> MGAKLAKTLQRFENKIKAGDYYEAHQTLRTIANRYVRSKSYEHAIELISQGALSFLKAKQGGSGTDLIFYLLEVYDLAEVKVDDISVARLVRLIAELDPSEPNLKDVITGMN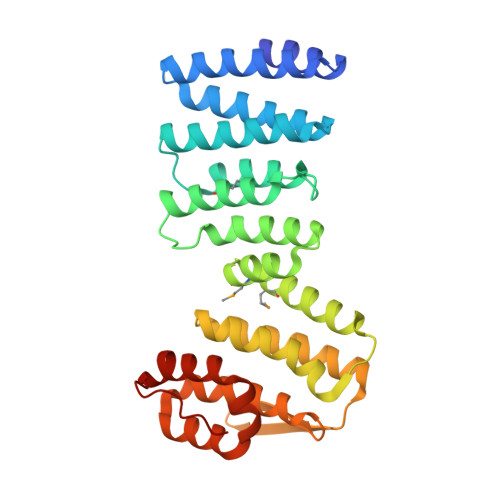NWSIKFSEYKFGDPYLHNTIGSKLLEGDFVYEAERYFMLGTHDSMIKYVDLLWDWLCQVDDIEDSTVAEFFSRLVFNYLFISNISFAHESKDIFLERFIEKFHPKYEKIDKNGYEIVFFEDYSDLNFLQLLLITCQTKDKSYFLNLKNHYLDFSQAYKSELEFLGQEYFNIVAPKQTNFL PfNCR1 is homologous to the human Niemann-Pick C1 (hNPC1) transporter. Our cryo-EM structure indicates that PfNCR1 is monomeric in form with overall dimensions of 110 Å × 75 Å × 55 Å. This transporter consists of a large membrane-spanning domain formed by 12 transmembrane helices (TM1 to TM12) and a large extension formed by two hydrophilic loops (loops 1 and 2), consistent with the signature of the resistance–nodulation–cell division (RND) superfamily of proteins. Therefore, our cryo-EM structure depicts that the PfNCR1 transporter contains two domains: the transmembrane PPM domain consisting of 12 TMs (TM1 to TM12) and the soluble PV domain composed of subdomains (PV1 and PV2). Combined, cryo-EM, Chl efflux assays, and molecular dynamics (MD) and targeted MD (TMD) simulations demonstrate that the PfNCR1 protein is capable of exporting Chls from the PPM to the parasitophorous vacuole (PV) to facilitate membrane homeostasis.

We also report the 2.98-Å cryo-EM structure of PfNCR1 bound with MMV009108, a potential PfNCR1 inhibitor that heightens the sensitivity of P. falciparum to saponin. The overall structure of PfNCR1-MMV009108 is very similar to that of PfNCR1-I. Superimposition of these two structures gives rise to an RMSD of 0.5 Å (for 871 Cα atoms), suggesting that the secondary structure of the transporter does not change significantly after inhibitor binding. The structure of PfNCR1-MMV009108 indicates that this transporter forms a channel (yellow) spanning the outer leaflet of the PPM domain and up to the PV domain. Similar to PfNCR1-I, this channel is broken into two halves. An extra density resembling Chl molecule is observed at the Chl binding site. The mode of binding for this Chl is the same as that found in the PfNCR1 structure without the addition of inhibitor. Our high-quality cryo-EM map also allows us to unambiguously depict the location of bound MMV009108. This inhibitor binds within the tunnel created by the PfNCR1 transporter. Within 4.5 Å from bound MMV009108, residues I63, L66, Y67, V486, P555, P556, T559, I625, F628, Y1105, A1108, F1109, F1305, I1368, I1369, K1434, F1436, T1437, and F1440 are engaged in anchoring this inhibitor molecule. On the basis of this structural information, the inhibition mechanism of MMV009108 appears to be due to a physical blockage of the tunnel formed by PfNCR1, disallowing this transporter to export Chl from the PPM of the parasite.

> MFVKNFIHKLKELKQKSLDKFANLLYDYGGYVYDRPCTFIICSLICCLLLTCGFYFKEHEKDIYKLYSISNSYAYETNETINDFFYKSRRCFILVESNVNLLKPKILRELQKFEEGTKDIEVDLSEINECKTNSELPPEQSHVAKELYKTLIQRSEENLKSGKINGSLFDYSDLDENGKSVLSLAGKENNDDTLIEGDNKNDEETSANNNNNEDDNNEDDNNEDDNNEDDNNENDNNNNNEDDNNNDDDDDEDNEEEDEEKQKSLREKLYRKIYEMLKKKKENIVLDENNPNVNFTDYKDDVFYPYQYIPPMLIKADRCKLQNVFGDKNLNIDLREASDGLKKQITYTLEDICEKKYGDCNFSSLFLYYEKGNGYIDYPIKVDNLDFYVNRRTYKEMMFKGILGNMVYEKSGSKYIIKSANAIMTVIPLLNSHTYEPYALAYEKKLIDYVRFYNLDDIIQDEETNDDNDPFIRFHVFTDRSLEDEVDRISKIDNLTRLLLLIGVLLIFMYALFNNVTSVLYRSKPLCAVMGIFCGFLGFLSGSGFLYFLGVKSVPPAETVPFLVIGVGVDDVFVILNSYSLLFMVKDNKKRIQMCLKDSALAITVTTLTNIIAFLISAISPFYSICAFSLFTASSLFFGYLMVLTFLLSFLCIEAKLEKKKRNIFTGTFHLFRSIFMKSSKKNKKENKENNIHDDGDNDNDEKKKDLSLEVKNNEDDYENISIYEWIHNLYLFEESINKKKKNAALVYASNNGMSSNLNNVNEDGFPNPSKIVSMEDVKKRNIKKDDAYINKEDEEGGGYYNKDDNKKKDILGKKQKKNNNNVTLVSKKGEDNELDVYYENLDEKTNDKYKMNNIKSSKLKYDNDKKDGAIINNRPSSDEEYKEEKDKNKINILNDVFNDITIKPNENILLDRGDVIKSSGYDSSYNDLQSSSLPNPSSNEVLNKTTMVYNETDLKDNKKEIKSSKKNVKDIKKSDMIHDDTYDIINSNNKNILLSSNEINNNSNNTNKFNNNSTELATKDTQQFINGHDKNIYLLSSHDNALFYKYIYEEPKGNIGKYFRSLVKNYYVPFLSSRFGKTIVYIMFTIIIAMSIYGCTLMKKGIKYDKAFPVDSYVRRFTTAKIKYFPDFGDFIEVYYFDKHFINKYRGLEKNTKEAASSFLYSDLTDRQIMNSPKINKNVHWENTNLQEELINMHNTLESQEFVTSVANGFTFFLNKNKSSLRKENPQEFYEIFANWLKKDFVGNLFKNDFVFLNGKLVAWRFHYFQKNVDDSEISSKWLKACKQITKLENHNVQMVCFHLSSIFNETDESIIEVTLINLGITILTILVVTAYIIKGFYSCVIIALIIFLIDLCIFGFMCLCGITMNIISMVILVLSVGFSIDHTSHIVQAFSHSMGRTRDEKMKESLHLMIGPVLHSGLSTWFVISTLFFSNKDFTVIFFQTLSLVLFFSITFSSMFLPVLLSSFGPLH>[4x]GMRRGLVIVGHGSQLNHYREVMELHRKRIEESGAFDEVKIAFAARKRRPMPDEAIREMNCDIIYVVPLFISYGLHVTEDLPDLLGFPRGRGIKEGEFEGKKV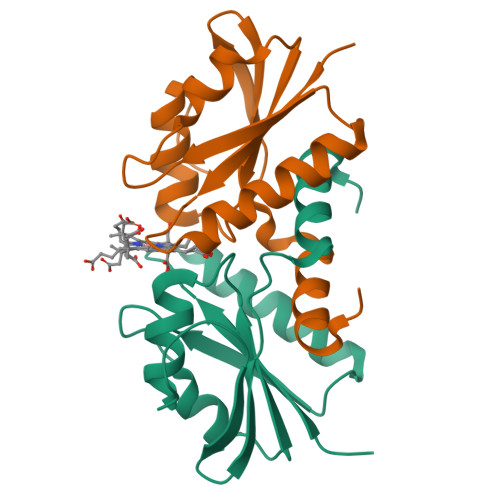VICEPIGEDYFVTYAILNSVFRIGRDGKGEE> PISPIET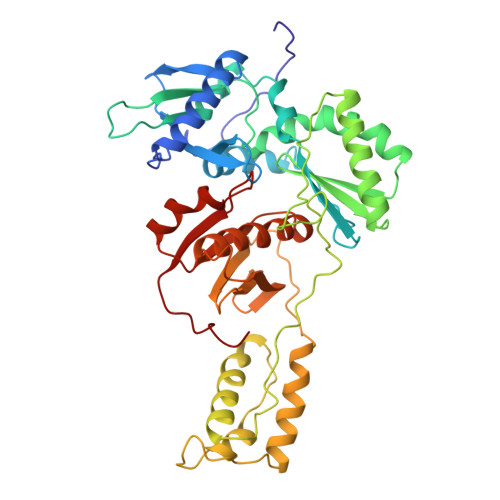VPVKLKPGMDGPKVKQWPLTEEKIKALVEICTEMEKEGKISKIGPENPYNTPVFAIKKKDSTKWRKLVDFRELNKRTQDFWEVQLGIPHPAGLKKKKSVTVLDVGDAYFSVPLDEDFRKYTAFTIPSINNETPGIRYQYNVLPQGWKGSPAIFQSSMTKILEPFRKQNPDIVIYQYMDDLYVGSDLEIGQHRTKIEELRQHLLRWGLTTPDKKHQKEPPFLWMGYELHPDKWTVQPIVLPEKDSWTVNDIQKLVGKLNWASQIYPGIKVRQLSKLLRGTKALTEVIPLTEEAELELAENREILKEPVHGVYYDPSKDLIAEIQKQGQGQWTYQIYQEPFKNLKTGKYARTRGAHTNDVKQLTEAVQKITTESIVIWGKTPKFKLPIQKETWETWWTEYWQATWIPEWEFVNTPPLVKLWY> MSLRIGVIGTGKIGKEHINRITNKLSGAEIVAVTSVNQEAAQKVVEQYQLNATVYPNDDSLLADENVDAVLVTSWGPAHESSVLKAIKAQKYVFCEKPLA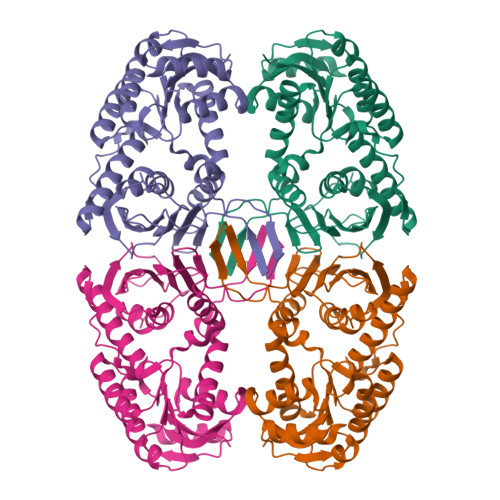TTAEGCMRIVEEEIKVGKRLVQVGFMRRYDSGYVQLKEALDNHVIGEPLMIHCAHRNPTVGDNYTTDMAVVDTLVHEIDVLHWLVNDDYESVQVIYPKKSKNALPHLKDPQIVVIETKGGIVINAEIYVNCKYGYDIQCEIVGEDGIIKLPEPSSISLRKEGRFSTDILMDWQRRFVAAYDVEIQDFIDSIQKKGEVSGPTAWDGYIAAVTTDACVKAQESGEKEKVELKEKPEFYQ>MTIIINVRERIEEWKIRIAAGFIREGKLVAFPTETVYGLGANALDENAVKRIFEAKGRPADNPLIIHIASFEQLEVLAKEIPEEAEMLAKRFWPGPLTLVLPKSEVVPRVITGGLDTVAVRMPAHEIALKLIELSERPIAAPSANISGKPSPTSAHHVAEDFYGKIECIIDGGETRIGVESTVIDLTEWPPVLLRPGGLPLEEIEKVIGEIRIHPAVYGKSVDTAKAPGMKYRAAAPSAEVIVVEGPRDKVRRKIEELIAKFKEEGKKVGVIGSGSYDADEVFYLGDTVEEIARNLFKALRHMDRTGVDVILAEGVEEKGLGLAVMNRLRKASGYR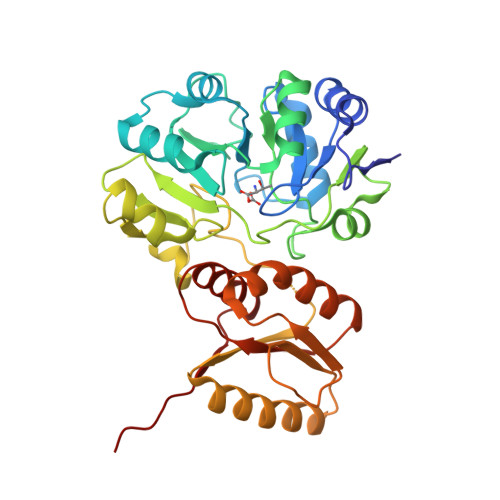IIKVHHHHHH[2x]> MGSDKIHHHHHHNTPREVTLHFLRTAGHPLTRWALQRQPPSPKQLEEEFLKIPSNFVSPEDLDIPGHASKDRYKDILPNPQSRVCLGRA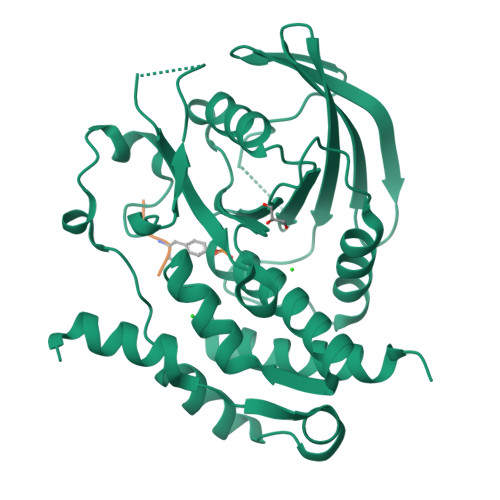QSQEDGDYINANYIRGYDGKEKVYIATQGPMPNTVSDFWEMVWQEEVSLIVMLTQLREGKEKCVHYWPTEEETYGPFQIRIQDMKECPEYTVRQLTIQYQEERRSVKHILFSAWPDHQTPESAGPLLRLVAEVEESPETAAHPGPIVVHSSAGIGRTGCFIATRIGCQQLKARGEVDILGIVCQLRLDRGGMIQTAEQYQFLHHTLALYAGQLPEEPSP;> LDEYVATR2-[(3-chloro-4-methoxybenzyl)amino]ethanesulfonic 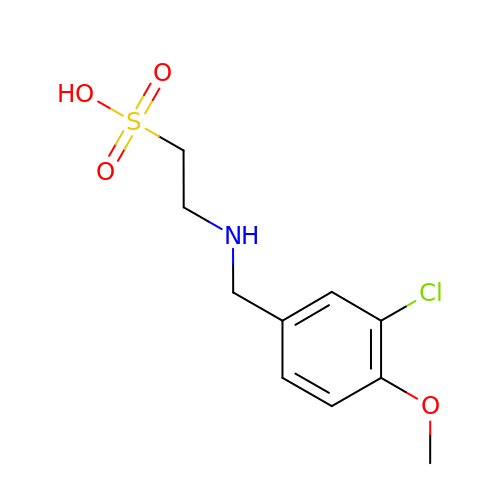acid | C10 H14 Cl N O4 S | BLSMHIDLTUGMQS-UHFFFAOYSA-N(3S)-5'-chloro-5-(cyclobutylmethyl)-2',3',4,5-tetrahydro-2H-spiro[1,5-benzoxazepine-3,1'-indene]-7-carboxylic acid | C23 H24 Cl N O3 | 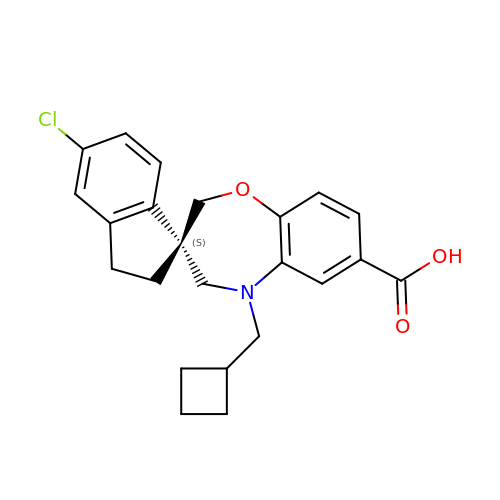YLXRDIJLTBHLLJ-QHCPKHFHSA-N>[6x]MERTFLMIKPDAVQRN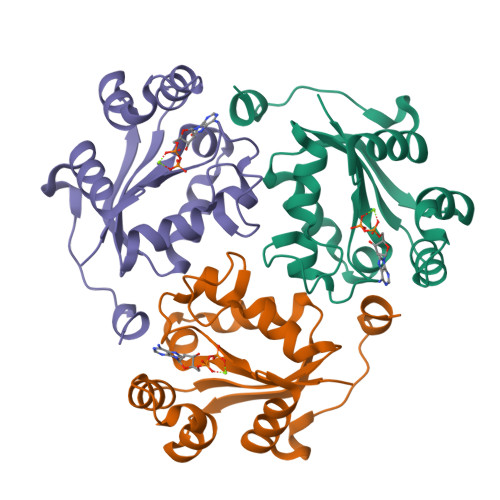LIGEVISRIERKGLKLVGGKLMQVPMELAETHYGEHQGKPFYNDLISFITSAPVFAMVVEGEDAVNVSRHIIGSTNPSEASPGSIRGDLGLTVGRNIIHGSDSLESAEREINLWFNENEITSYASPRDAWLYELEHHHHHH> AEIYNKDGNKVDLYGKAVGLHYFSKGNGENSYGGNGDMTYARLGFKGETQINSDLTGYGQWEYNFQGNNSEGADAQTGNKTRLAFAGLKYADVGSFDYGRNYGVVYDALGYTDMLPEFGGDTAYSDDFFVGPVGGVATYRNSNFFGLVDGLNFAVQ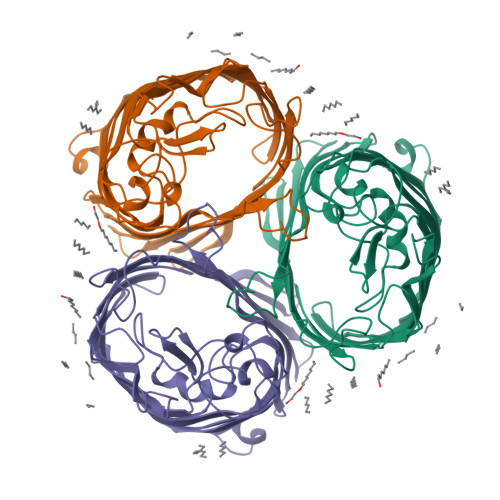YLGKNERDTARRSNGDGVGGSISYEYEGFGIVGAYGAADRTNLQEAQPLGNGKKAEQWATGLKYDANNIYLAANYGETRNATPITNKFTNTSGFANKTQDVLLVAQYQFDFGLRPSIAYTKSKAKDVEGIGDVDLVNYFEVGATYYFNKNMSTYVDYIINQIDSDNKLGVGSDDTVAVGIVYQF>SMTNNKYYTEENKKKVWKKHMIVLKFLEQPGISEAYLNYLQEEIHNDEWIGFENEFFEELTGKPVINVGDKIKATKQYSAVH[2x]

Here we determined that the arbitrium system in Bacillus subtilis phage phi3T modulates the bacterial toxin–antitoxin system MazE–MazF to regulate the phage life cycle. AimX also inhibits the function of phi3T_93, a protein that promotes lysogeny by binding to MazE and releasing MazF. In all structures, phi3T_93 shows an identical all-helices fold composed of a longer N-terminal helix (α1), followed by two shorter helices (α2 and α3) connected by a long unstructured loop forming a V-like shape. The α1 helices of two phi3T_93 monomers interact, resulting in a W-shaped tight and globular dimer that displays two shallow grooves, one across each side of the dimer molecule.

We obtained the structure of phi3T_93 alone (wt and its N-terminal His-tagged version; His-phi3T_93) and in complex with AimX. Size exclusion chromatography coupled to multi-angle light scattering (SEC–MALS) analysis confirmed the phi3T_93 dimeric organization in solution. We hypothesize that phi3T_93 promotes lysogeny by binding AimX and MazE, reducing the amount of antitoxins that can block MazF activity.> PISPIETVPVKLKPGMDGPKVKQWPLTEEKIKALVEICTEMEKEGKISKIGPENPYNTPVFAIKKKDSTKWRKLVDFRELNKRTQDFWEVQLGIPHPAGLKKKKSVTVLDVGDAYFSVPLDEDFRKYTAFTIPSINNETPGIRYQYNVLPQGWKGSPAIFQSSMTKILEPFKKQNPDIVIYQYMDDLYVGSDLEIGQHRTKIEELRQHLLRWGLTTPDKKHQKEPPFLWMGYELHPDKWTVQPIVLPEKDSWTVNDIQKLVGKLNWASQIYPGIKVRQLCKLLRGTKALTEVIPLTEEAELELAENREILKEPVHGVYYDPSKDLIAEIQKQGQGQWTYQIYQEPFKNLKTGKYARMRGAHTNDVKQLTEAVQKITTESIVIWGKTPKFKLPIQKETWETWWTEYWQATWIPEWEFVNTPPLVKLWYQL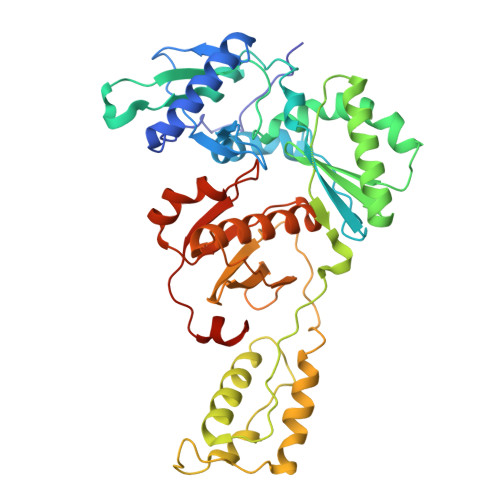EKEPIVGAETF>MKKLLTVMTMAVLTAGTLLLPAQSVTPAAHAVQISNSERELPFKAKHAYSTISQLSEAIGPRIAGTAAEKKSALLIASSMRKLKLDVKVQRFNIPDRLEGTLSSAGRDILLQAASGSAPTEEQGLTAPLYNAGLGYQKDFTADAKGKIALISRGDLTYYEKAKNAEAAGAKAVIIYNNKESLVPMTPNLSGNKVGIPVVGIKKEDGEALTQQKEATLKLKAFTNQTSQNIIGIKKPKNIKHPDIVYVTAHYDSVPFSPGANDNGSGTSVMLEMARVLKSVPSDKEIRFIAFGAEELGLLGSSHYVDHLS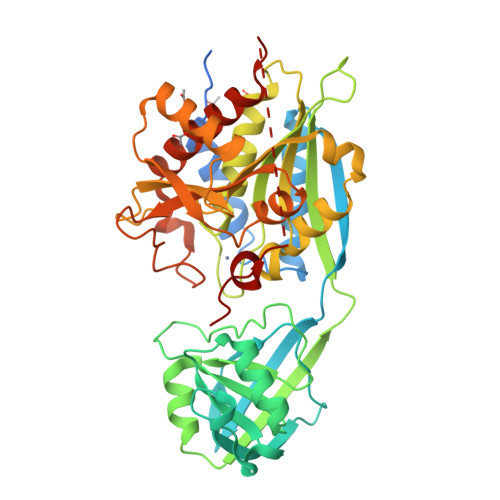EKELKRSEVNFNLDMVGTSWEKASELYVNTLDGQSNYVWESSRTAAEKIGFDSLSLTQGGSSDHVPFHEAGIDSANFIWGDPETEEVEPWYHTPEDSIEHISKERLQQAGDLVTAAVYEAVKKEKKPKTIKKQMKAKASDIFEDIK[3x]> QYDDDWQYEDCKLARGGPPATIVAIDEESRNGTILVDNMLIKGTAGGPDPTI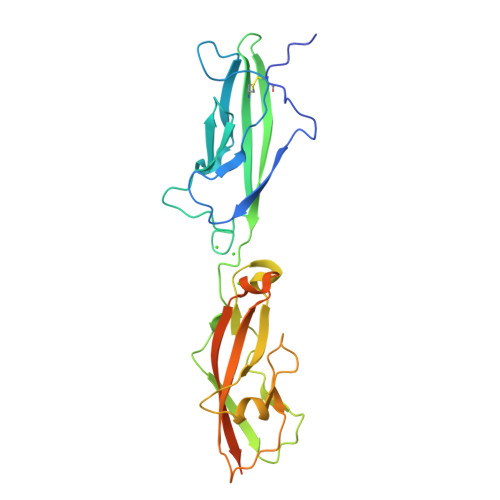ELSLKDNVDYWVLLDPVKQMLFLNSTGRVLDRDPPMNIHSIVVQVQCVNKKVGTVIYHEVRIVVRDRNDNSPTFKHESYYATVNELTPVGTTIFTGFSGDNGATDIDDGPNGQIEYVIQYNPEDPTSNDTFEIPLMLTGNVVLRKRLNYEDKTRYYVIIQANDRAQNLNERRTTTTTLTVDVLDGDDGLNDIFEAQKIEWHELEHHHHHH>[2x]MHHHHHHVSHDDLMLALALADRADELTRVRFGALDLRIDTKPDLTPVTDADRAVESDVRQTLGRDRPGDGVLGEEFGGSTTFTGRQWIVDPIDGTKNFVRGVPVWASLIALLEDGVPSVGVVSAPALQRRWWAARGRGAFASVDGARPHRLSVSSVAELHSASLSFSSLSGWARPGLRERFIGLTDTVWRVRAYGDFLS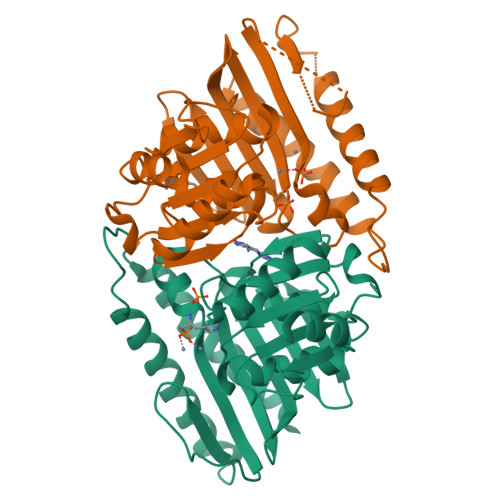YCLVAEGAVDIAAEPQVSVWDLAALDIVVREAGGRLTSLDGVAGPHGGSAVATNGLLHDEVLTRLNAG>[4x]MASAEDVVVVNKQVLLKHFIPEGAPKETDMELVTTGTIRLRVPEGSNAVLLKNLYLSCDPYMRMR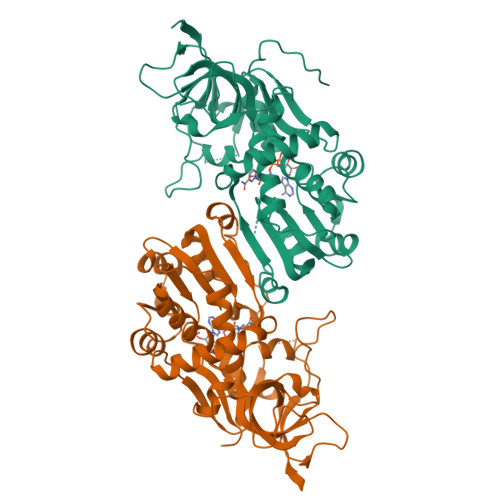MTKHEEASYVDDFVPGAPITGFGVGKVVDSSHPDFKTGDYVWGLIGWEEYSLITKPQGLFKIHHTEIPLSYYTGILGMVGLTAYVGFYDICSPKKGERVFVSAAAGAVGQIVGQFAKQFGCYVVGSAGSDEKVNLLKTKFGFDEAFNYKKEPDLTKALKRYFPEGIDIYFENVGGPMLEAVLHNMRIKGRIAACGMISQYNLEKPEGVHNLFLIVGKRIRLEGFLVFDHYGSYPEFEEKVVQLIKEEKIKYLEDIVEGLENAPAALIGLFEGRNVGKQVVVVSREKGHHHHHH>[6x]MHHHHHHMREALGLIETK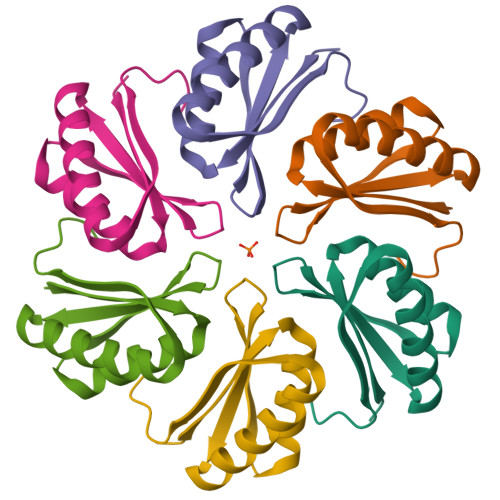GLVACIEAADAMCAAANVELIGYGNVGSGLVTAMVKGDVGAVNAAVDSGVEAARRIGEVVTSRVIARPHNDIEKIASQHKA>[4x]HHHHHHDITFRNIRFRYKPDSPVILDNINLSIKQGEVIGIVGRSGSGKSTLTKLIQRFYIPENGQVLIDGHDLALADPNWLRRQVGVVLQDNVLLNRSIIDNISLANPGMSVEKVI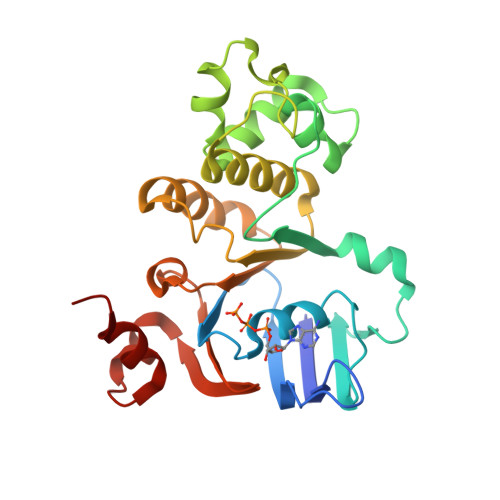YAAKLAGAHDFISELREGYNTIVGEQGAGLSGGQRQRIAIARALVNNPKILIFDEATSALDYESEHVIMRNMHKICKGRTVIIIAARLSTVKNADRIIVMEKGKIVEQGKHKELLSEPESLYSYLYQLQSD>ACCCGCAAGGCCGACGGC[2x];>[2x]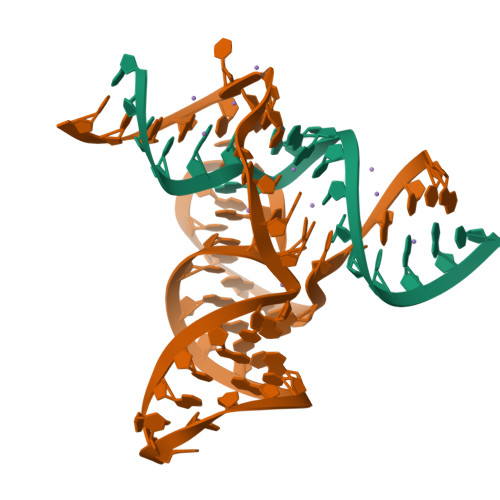GCCGCCGCUGGUGCAAGUCCAGCCACGCUUCGGCGUGGGCGCUCAUGGGU> M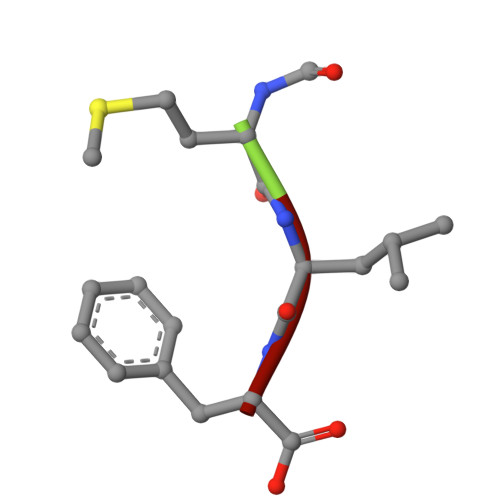LF1-(2-hydroxy-2,2-diphosphonoethyl)-3-phenylpyridinium | C13 H16 N O7 P2 | 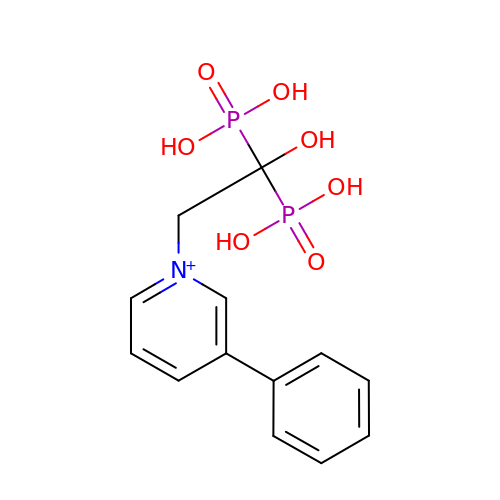ZYEONEYSNIUGRA-UHFFFAOYSA-O>MEMAISKAGRRLKAAKKVERKKIVSGPALPGKLADCVGQTREESELFIVEGDSAGGSAKQARDKNFQAIMPIRGKILNTWEVSSDEVLASQEVHDIAIAIGVDPGSDDLSELRYGKICILADADSDGLHIATLLCALFVKHFPALVEEGHLYVAMPPLFRIDIGKDVHYALDDEELETILKNVKGNKNPQITRFKGLGEMNAIQLRETTMDPNTRRLVQLDLDDAHLTAGLLDKLLAKKRAADRKQWLEQKGNLADITVEDKLTMTSLAHHATENRSVAEFTEQAYLNYAMYVIMDRALPHISDGLKPVQRRIVYAMSELGLKSSGKPKKSARTVGDVLGKYHPHGDSACYEAMVLMAQPFSYRYPLIEGQGNWGSPDDPKSFAAMRYTEAKLSAYSELLLSELGQGTSEWQDNFDGSLKEPITLPARVPNILLNGTTGIAVGMATDIPPHNLREVVKGTIALIRNPQTSDEKLAEYIPAPDLPTKAEIITPPEELLKIQTTGRGSYRMRAVYTIEKNEIVITELPYQVSGSKVITQIADQMQAKKLPLVVDVRDESDHENPTRLVIVLRSNRIDAEAVMSHLFATTDLESSYRVNLNMIGEDGRPQVKSIRRILLEWIEIRKKTVTRRLQYHLNRIEKRLHILAGLLIAYLDIDTVIRIIREEDQPKPVLMEHFNIDEIQAEAILELKLRHLAKLEEMEIRHEQDELSAKAAIIREQLENPESLKNLIISELKEDAKKFGDERR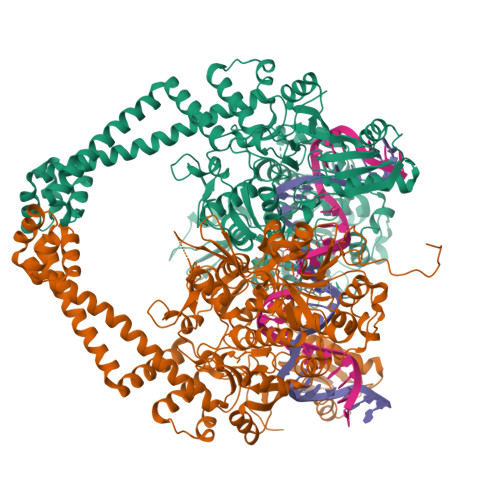SPIVARAEAVQIKEQDLMPAET[2x]1,5-anhydro-2,3-dideoxy-3-[(5S)-5H-imidazo[5,1-a]isoindol-5-yl]-D-threo-pentitol 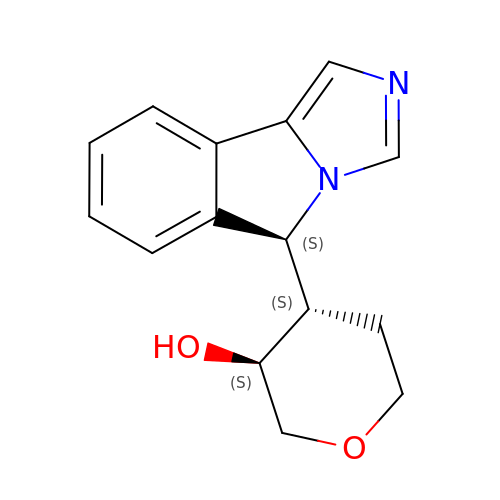| C15 H16 N2 O2 | WENBZVXOQQBSHR-BPLDGKMQSA-N> XAAAA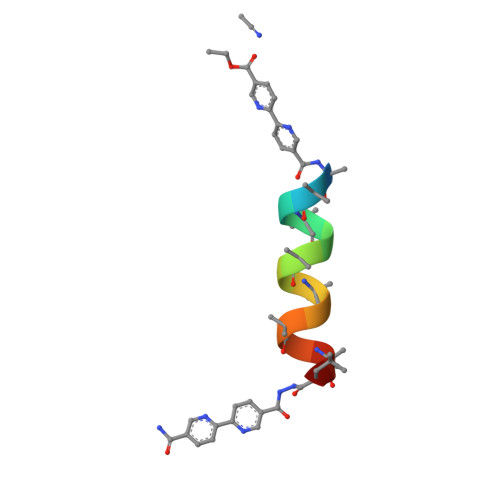LAAALAQALX>[2x]GHMFFSKDEKNPIKRALQGELLQNEPFIQLCTKIENYLMDTEAVNEQLIELNEQLTMRLKEKGLKPGEKGATKQLRTLIQEILTEAGFREGMLQTIGNKPLA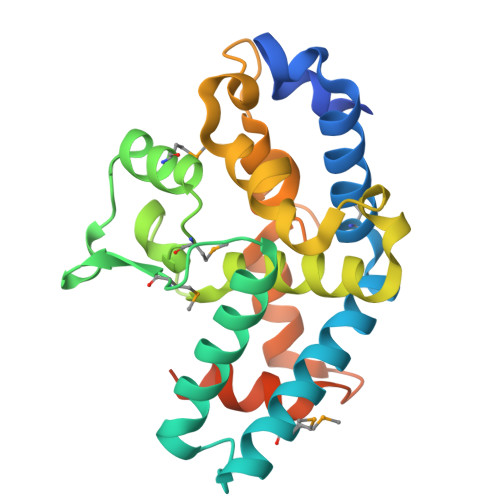AADFMFLVSSGFMLKDSSLRASSHGELTHAIQWCLIILKRKKDSSFLENIPTSEICDRIYKKLGHQDSSNPNYPFTCWDVLIDKLGEIDSRSPEWLSDHIQNDEDQIFPVLREVIKNRTEKGKTEENKGKLQKKLENGS> ECR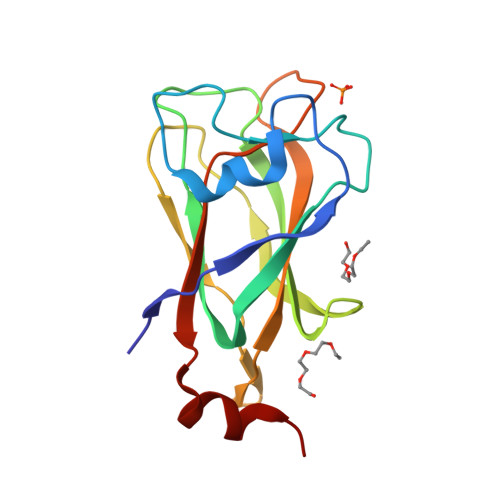LLPYALHKWSSFSSTYLPENILVDKPNDQSSRWSSESNYPPQYLILKLERPAIVQNITFGKYEKTHVCNLKKFKVFGGMNEENMTELLSSGLKNDYNKETFTLKHKIDEQMFPCRFIKIVPLLSWGPSFNFSIWYVELSGIDDPDIVQPCLNW>GGSGERKISRIHLVSEPSITHFLQVSWEKTLESGFVITLTDGHSAWTGTVSESEISQEADDMAMEKGKYVGELRKALLSGAGPADVYTFNFSKESCYFFFEKNLKDVSFRLGSFNLEKVENPAEVIRELICYCLDTTAENQAKNEHLQLEFNQIKAEIERKLAEKDEEM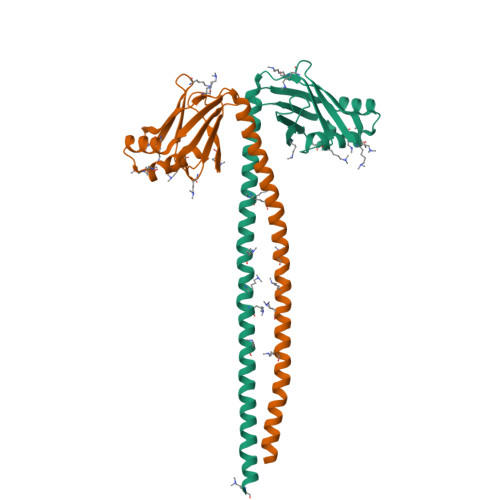EQAKRNHLRVVDSLQTSLDAETRSRNEALRVKKKMEGDL[4x]> GSMAVDGGCGDTGDWEGRWNHVKKFLERSGPFTHPDFEPSTESLQFLLDTCKVLVIGAGGLGCELLKNLALSGFRQIHVIDMDTIDVSNLNRQFLFRPKDIGRPKAEVAAEFLNDRVPNCNVVPHFNKIQDFNDTFYRQFHIIVCGLDSIIARRWINGMLISLLNYEDGVLDPSSIVPLIDGGTEGFKGNARVILPGMTACIECTLELYPPQVNFPMCTIASMPRLPEHCIEYVRMLQWPKEQPFGEGVPLDGDDPEHIQWIFQKSLERASQYNIRGVTYRLTQGVVKRIIPAVASTNAVIAAVCATEVFKIATSAYIPLNNYLVFNDVDGLYTYTFEAERKENCPACSQLPQN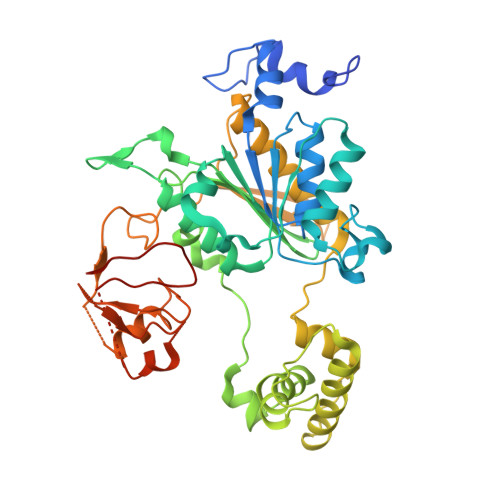IQFSPSAKLQEVLDYLTNSASLQMKSPAITATLEGKNRTLYLQSVTSIEERTRPNLSKTLKELGLVDGQELAVADVTTPQTVLFKLHFTS1,6-dimethylpyrimido[5,4-e][1,2,4]triazine-5,7(1H,6H)-dione 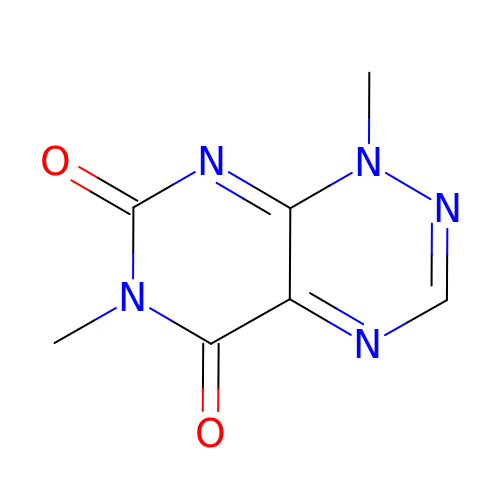| C7 H7 N5 O2 | SLGRAIAQIAUZAQ-UHFFFAOYSA-N>[2x]MSKLPQVKALYPYTAANDEELSFKVGDIITILEKDEGWWKGELNG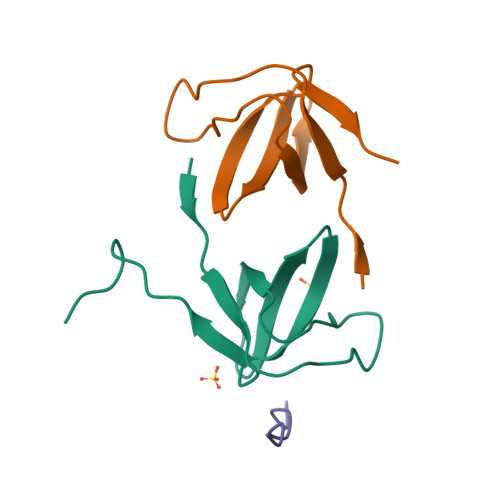QEGWIPNNYVKEILEHHHHHH;> KVAPPIPHR>[8x]MTYTVGMYLAERLVQI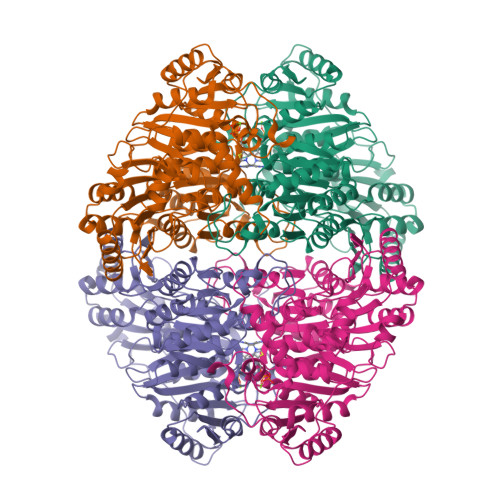GLKHHFAVAGDYNLVLLDQLLLNKDMKQIYCCNELNCGFSAEGYARSNGAAAAVVTFSVGAISAMNALGGAYAENLPVILISGAPNSNDQGTGHILHHTIGKTDYSYQLEMARQVTCAAESITDAHSAPAKIDHVIRTALRERKPAYLDIACNIASEPCVRPGPVSSLLSEPEIDHTSLKAAVDATVALLEKSASPVMLLGSKLRAANALAATETLADKLQCAVTIMAAAKGFFPEDHAGFRGLYWGEVSNPGVQELVETSDALLCIAPVFNDYSTVGWSAWPKGPNVILAEPDRVTVDGRAYDGFTLRAFLQALAEKAPARPASAQKSSVPTCSLTATSDEAGLTNDEIVRHINALLTSNTTLVAETGDSWFNAMRMTLPRGARVELEMQWGHIGWSVPSAFGNAMGSQDRQHVVMVGDGSFQLTAQEVAQMVRYELPVIIFLINNRGYVIEIAIHDGPYNYIKNWDYAGLMEVFNAGEGHGLGLKATTPKELTEAIARAKANTRGPTLIECQIDRTDCTDMLVQWGRKVASTNARKTTLALEHHHHHH> MNILLVSQCEKRALSETRRILDQFAERRGERTWQTPITQAGLDTLRRLLKKSARRNTAVACHWIRGRDHSELLWIVGDASRFNAQGAVPTNRTCRDILRKEDENDWHSAEDIRLLTVMAALFHDIGKASQAFQAKLRNRGKPMADAYRHEWVSLRLFEAFVGPGSSDEDWLRRLADKRETGDAWLSQLARDDRQSAPPGPFQKSRLPPLAQAVGWLIVSHHRLPNGDHRGSASLARLPAPIQSQWCGARDADAKEKAACWQFPHGLPFASAHWRARTALCAQSMLERPGLLARGPALLHDSYVMHVSRLILMLADHHYSSLPADSRLGDPNFPLHANTDRDSGKLKQRLDEHLLGVALHSRKLAGTLPRLERQLPRLARHKGFTRRVEQPRFRWQDKAYDCAMACREQAMEHGFFGLNLASTGCGKTLANGRILYALADPQRGARFSIALGLRSLTLQTGQAYRERLGLGDDDLAILVGGSAARELFEKQQERLERSGSESAQELLAENSHVHFAGTLEDGPLREWLGRNSAGNRLLQAPILACTIDHLMPASESLRGGHQIAPLLRLMTSDLVLDEVDDFDIDDLPALSRLVHWAGLFGSRVLLSSATLPPALVQGLFEAYRSGREIFQRHRGAPGRATEIRCAWFDEFSSQSSAHGAVTSFSEAHATFVAQRLAKLEQLPPRRQAQLCTVHAAGEARPALCRELAGQMNTWMADLHRCHHTEHQGRRISFGLLRLANIEPLIELAQAILAQGAPEGLHVHLCVYHSRHPLLVRSAIERQLDELLKRSDDDAAALFARPTLAKALQASTERDHLFVVLASPVAEVGRDHDYDWAIVEPSSMRSIIQLAGRIRRHRSGFSGEANLYLLSRNIRSLEGQNPAFQRPGFETPDFPLDSHDLHDLLDPALLARIDASPRIVEPFPLFPRSRLVDLEHRRLRALMLADDPPSSLLGVPLWWQTPASLSGALQTSQPFRAGAKERCYALLPDEDDEERLHFSRYEEGTWSNQDNLLRNLDLTYGPRIQTWGTVNYREELVAMAGREDLDLRQCAMRYGEVR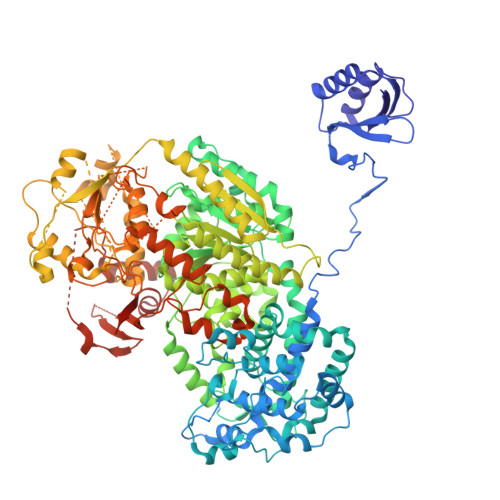LRENTQGWSYHPYLGFKKYN1-tert-butyl-3-(3-chlorophenoxy)-1H-pyrazolo[3,4-d]pyrimidin-4-amine | C15 H16 Cl 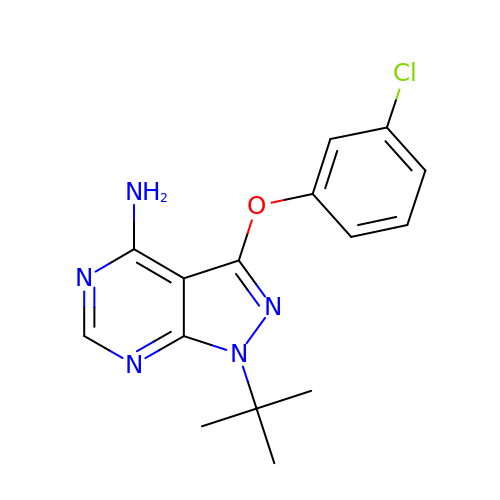N5 O | FOCSESRERLFAOP-UHFFFAOYSA-N>[2x]CGCGGATU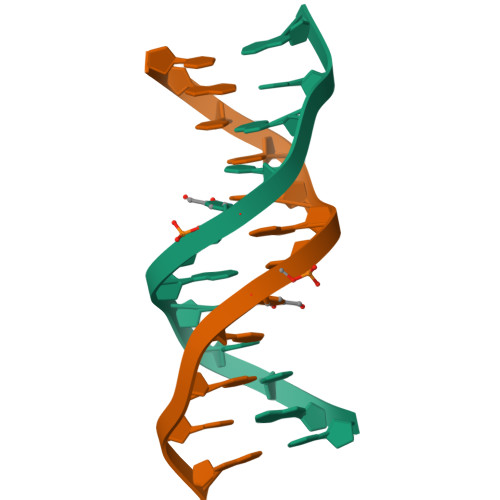CGCG7-hydroxy-N-[(2S)-1-hydroxypropan-2-yl]-5-phenylpyrazolo[1,5-a]pyrimidine-3-carboxamide 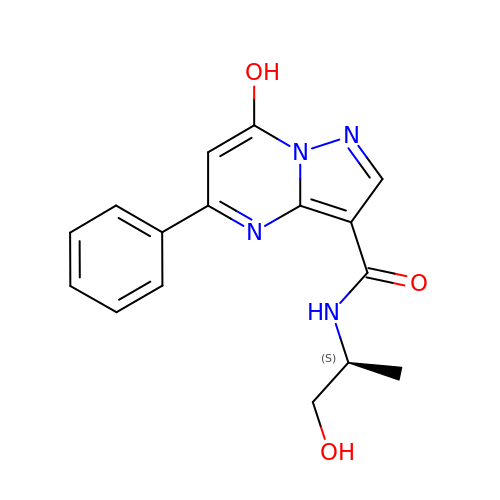| C16 H16 N4 O3 | HXHYZXUIKFXLHE-JTQLQIEISA-N>[2x]SMKLDIKKTFSNRSDRVKGIDFHPTEPWVLTTLYSGRVEIWNYETQVEVRSIQVTETPVRAGKFIARKNWIIVGSDDFRIRVFNYNTGEKVVDFEAHPDYIRSIAVHPTKPYVLSGSDDLTVKLWNWENNWALEQTFEGHEHFVMCVAFNPKDPSTFASGCLDRTVKVWSLGQSTPNFTL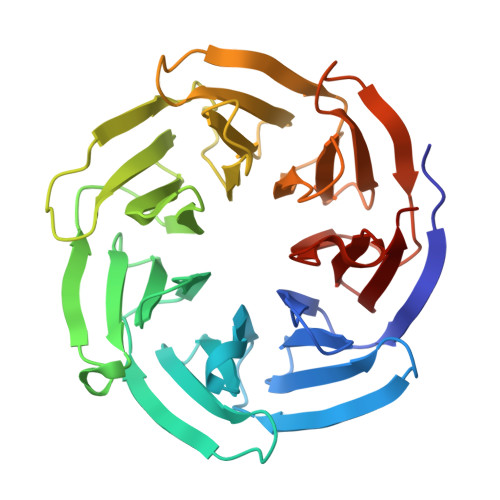TTGQERGVNYVDYYPLPDKPYMITASDDLTIKIWDYQTKSCVATLEGHMSNVSFAVFHPTLPIIISGSEDGTLKIWNSSTYKVEKTLNVGLERSWCIATHPTGRKNYIASGFDNGFTVLSLG>DLTNLVAEPFAKLEQDFGGSIGVYAMDTGSGATVSYRAEERFPLCSSFKGFLAAAVLARSQQQAGLLDTPIRYGKNALVPWSPISEKYLTTGMTVAELSAAAVQYSDNAAANLLLKELGGPAGLTAFMRSIGDTTFRLDRWEL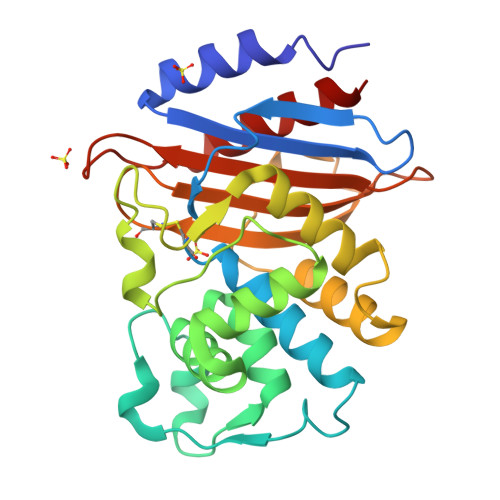ELNSAIPGDARDTSSPRAVTESLQKLTLGSALAAPQRQQFVDWLKGNTTGNHRIRAAVPADWAVGDKTGTCGVYGTANDYAVVWPTGRAPIVLAVYTRAPNKDDKHSEAVIAAAARLALEGLG[4x]> LGSSNDN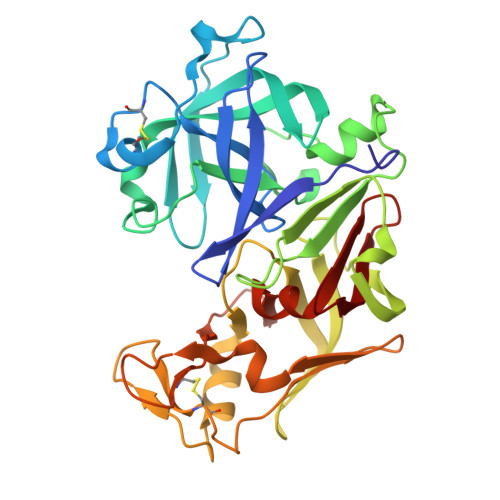IELVDFQNIMFYGDAEVGDNQQPFTFILDTGSANLWVPSVKCTTAGCLTKHLYDSSKSRTYEKDGTKVEMNYVSGTVSGFFSKDLVTVGNLSLPYKFIEVIDTNGFEPTYTASTFDGILGLGWKDLSIGSVDPIVVELKNQNKIENALFTFYLPVHDKHTGFLTIGGIEERFYEGPLTYEKLNHDLYWQITLDAHVGNISLEKANCIVDSGTSAITVPTDFLNKMLQNLDVIKVPFLPFYVTLCNNSKLPTFEFTSENGKYTLEPEYYLQHIEDVGPGLCMLNIIGLDFPVPTFILGDPFMRKYFTVFDYDNHSVGIALAKKNL cyclohexanecarboxylic acid | C7 H12 O2 | 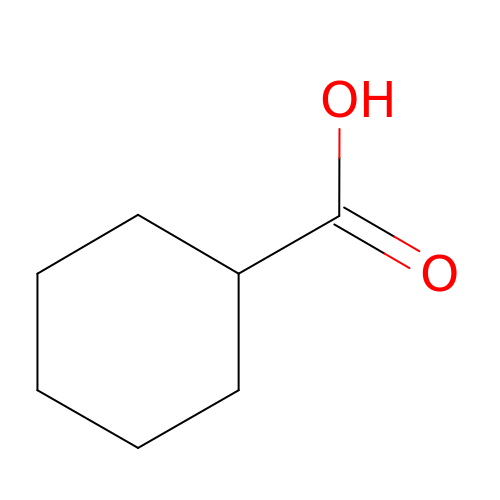NZNMSOFKMUBTKW-UHFFFAOYSA-N> Q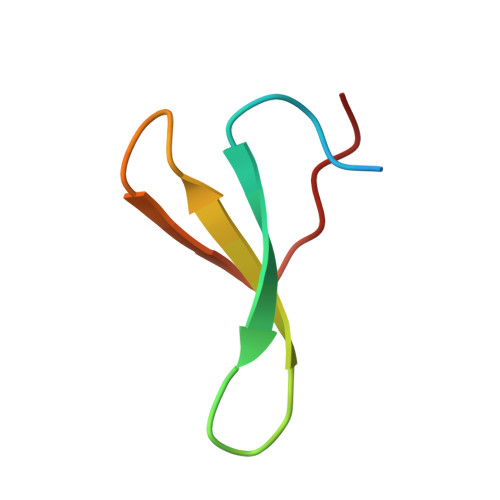PHMPGLPSGWEERKDAKGRTYYVNHNNRTTTWTRPIM piperlongumine | C17 H19 N O5 | 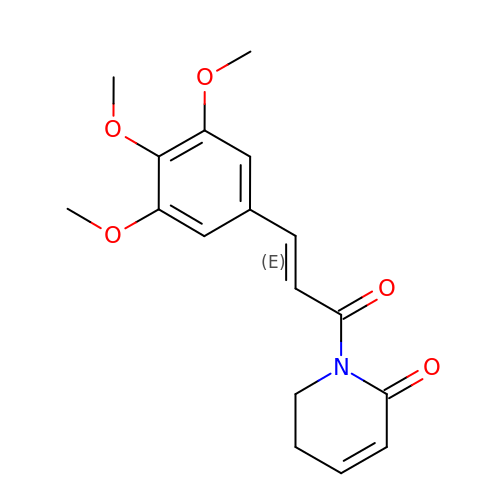VABYUUZNAVQNPG-BQYQJAHWSA-N> MTCNIKNGRCEQ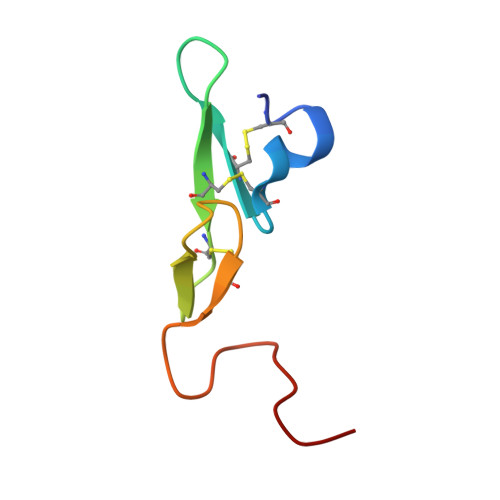FCKNSADNKVVCSCTEGYRLAENQKSCEPAVPFPCGRVSVSQ> GHMKPKRDLMADFTKWFVTGDGGIMEEFTEETLRHLLWDVWQRHQREEAERKRKAEEEESWRLARE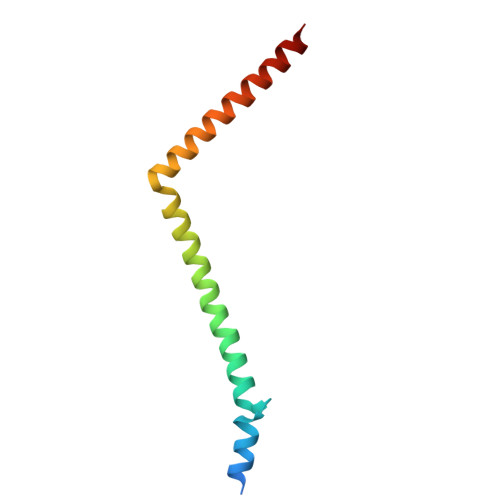HLTHRLQVKYFYRWREKARALAT> MTLGTNQVSKTHSFMTVSLIELWERFGYYGMQALIVYFMVQRLGFDDSRANLVWSACAALIYVSPAIGGWVGDKILGTKRTMLLGAGILSVGYALMTVPTENTWFMFSALGVIVVGNGLFKPNAGNLVRKIYEGDDSKIDSAFTIYYMAVNVGSTFSMLLTPWIKDYVNAQYGNEFGWHAAFAVCCVGILVGLGNYALMHKSLANYGSEPDTRPVNKKSLAIVLALAALSVVASAIILEYEDVARVFVYAAGVAVLGIFFHLIRTSEPSERAGLIAALILTVQTVFFFIFYQQMSTSLALFALRNVDWDFQVFGTHLWTWSPAQFQALNPIWIMVLSPVLAWSYSWAGRNNKDFSIAAKFALGFAVVAIGFFIYGFAGQFAVNGKTSSWVMIWGYASYSLGELLVSGLGLAMIARYVPARMGGFMMGAYFVASGISQYLGGVVANFASVPQDLVDPLQTLPVYTNLFNKLGVAAVVCTIIALAVLPLMRRLTESHHAHSSIENNAAASLRDVKAEQLESSGENLYFQ

Proton-dependent oligopeptide transporters (POTs) belong to the major facilitator superfamily (MFS) and transport short-chain peptides from the extracellular environment into the target cell. Previously reported structures revealed that the bacterial POTs possess 14 helices, of which H1–H6 and H7–H12 constitute the typical MFS fold and the residual two helices, HA and HB, are inserted between H6 and H7. PepTSo2 from Shewanella oneidensis is a unique POT transporter that has been reported to assemble as a 200 kDa tetramer in the detergent-solubilized form. In this study, a combination of X-ray crystallographic and single-particle cryo-EM analyses revealed the species-specific tetramer formation mechanism of PepTSo2, in which the two asparagine residues in H12 and the unpreserved ECL play key roles.

To further improve the resolution, we tried to crystallize tetrameric PepTSo2 using the LCP method at protein concentrations of 20, 45 and 75 mg ml−1. Microcrystals of PepTSo2 were obtained using a 45 mg ml−1 sample under multiple conditions containing PEG 200 as a precipitant. Since the size of the crystals was too small and data collection from a single crystal was impossible, small wedge data were collected from microcrystals using the microfocus beam at BL32XU at SPring-8, Hyogo, Japan and were combined using the multi-crystal merging software KAMO. We finally determined structures of PepTSo2 from two different crystal forms at 3.5 and 3.9 Å resolution by merging small wedge data sets from multiple microcrystals. PepTSo2 forms a tetramer in both of the crystal forms, and the structures superimpose well (with an r.m.s.d. of 0.83 Å for all Cα atoms). All of the protomers in the tetramer adopted the inward-open conformation, in which a large central hydrophilic substrate-binding pocket faces the intracellular side of the membrane. The structural comparison shows that the present tetrameric structure superimposes well with the previously reported dimeric structure at the protomer level (r.m.s.d. of 1.1 Å for all Cα atoms). A slight movement of H12 was also observed, as in the previous structure, suggesting the importance of H12 for tetramer formation. Furthermore, the tetrameric assembly appears to be stabilized by hydrogen bonds between the asparagine residues in H12 and the unconserved extracellular loop (ECL), which was not well resolved in the previously determined low-resolution tetrameric structures.> GVYRVCVSTGASIYAGSKNKVELWLVGQHGEVELGSCLRPTRNKEEEFKVNVSKYLGSLLFVRLRKKHFLKEDAWFCNWISVQALGAAEDKYWFPCYRWVVGDGVQSLPVGTGCTTVGDPQGLFQKHREQELEERRKLYQWGS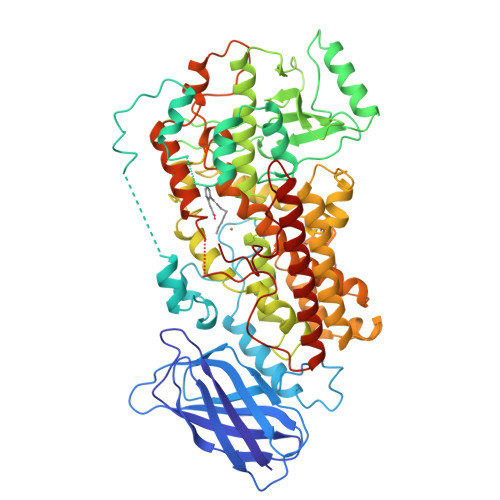WKEGLILNVAGSKLTDLPVDERFLEDKKIDFEASLAWGLAELALKNSLNILAPWKTLDDFNRIFWCGRSKLARRVRDSWQEDSLFGYQFLNGANPMLLRRSVQLPARLVFPPGMEELQAQLEKELKAGTLFEADFALLDNIKANVILYCQQYLAAPLVMLKLQPDGKLMPMVIQLHLPKIGSSPPPLFLPTDPPMVWLLAKCWVRSSDFQVHELNSHLLRGHLMAEVFTVATMRCLPSIHPVFKLIVPHLRYTLEINVRARNGLVSDFGIFDQIMSTGGGGHVQLLQQAGAFLTYRSFCPPDDLADRGLLGVESSFYAQDALRLWEIISRYVQGIMGLYYKTDEAVRDDLELQSWCREITEIGLQGAQKQGFPTSLQSVAQACHFVTMCIFTCTGQHSSIHLGQLDWFTWVPNAPCTMRLPPPTTKDATLETVMATLPNLKQSSLQMSIVWQLGRDQPIMVPLGQHQEEYFSGPEPRAVLEKFREELAIMDKEIEVRNEKLDIPYEYLRPSIVENSVAI>GAMAEGELGIVDIGALTLESGAVIDNVQIAVERWGELSPSRDNVVVVLHALTGDSHVAGPAGPNYPTPGWWDGVVGPGAAIDTRRWCAIATNVLGGCRGSTGPGSLHPDGKAWGSRFPAVTVRDQVRADLAALNAMGIHQVAAVVGGSMGGARALEWVIGHPETVRAGLILAVGARATADQIGTQSTQVAAIKADPNWQNGDYYGTGLKPDVGLQIARRFAHLTYRGEVELDTRFGNAPQDDENPLLGGRYAVESYLEYQGRKLVDRFDAGTYVTLTDSLSSHDVGRGRG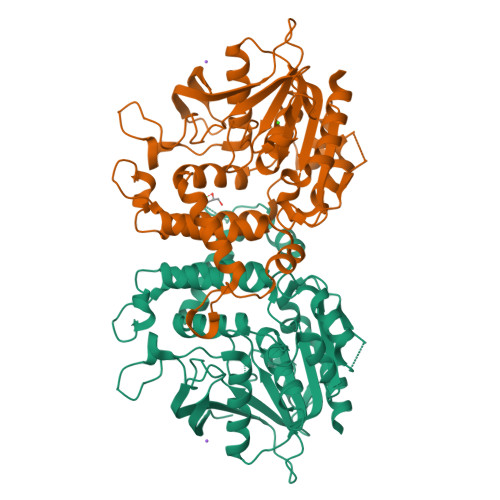GVEAALRSCEVPVVVGGFTSDRLYPLRLQEELAELMPGCRGLNVVESIYGHDGFLIETEAVGKLIRQTLELAS[2x]> MSQHINTVGYLEQKMFAAMVADNQMAMVMLNPKNLKASNGEEELAGQTWYWKVAPVATTQPLLKAFDVSVAATT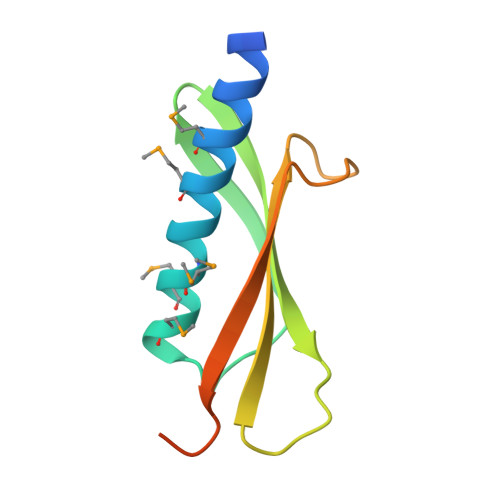QASPIITVRSYVASENLYFQGGGHHHHHH> MAHHHHHHMAIKPIYFDYMATTPVDPRVVEQMIKYLGPEGDFGNPASATHEYGRVASMAVEQARSQIAETINASPQEIVFTSGATEADNLAILGAARFYKNKGMHLVTMSTEHKAVLDSFHQLEKEGFQVTYLNPESDGLLDLEKLESALRLDTILVS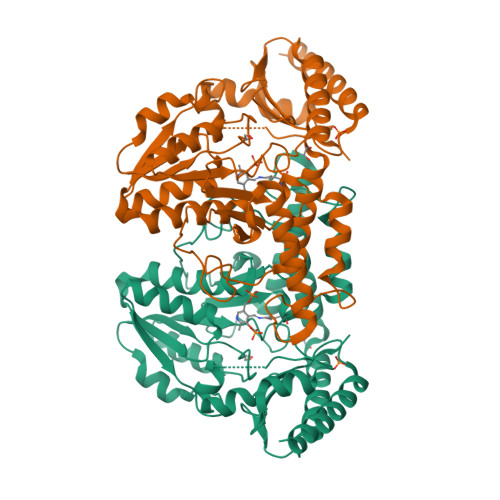VMHVNNEIGVIQDIASIGELLRNRGIIFHVDAAQSAGKLPIDLSQLSVDLMSFSAHKNYGPKGVGALYVRHKPRIRLQPLSYGGGHEGGLRSGTLPTHQIVGMGEAFAIAEADRIPEQTRILNLRKQLWDGIRHLPAIKLNGHEHRRIAGNLNVSFVGLNGDSLLFALSELAISTTSACSSASIQPSYVLRAIGLTDTEAQSTIRLSIGRFTSEVQIKKAIDIICTQVSRLHELSPL KaiC, a core protein of the cyanobacterial circadian clock, consists of an N-terminal CI domain and a C-terminal CII domain, and assembles into a double-ring hexamer upon binding with ATP. KaiC rhythmically phosphorylates and dephosphorylates its own two adjacent residues Ser431 and Thr432 at the CII domain with a period of ∼24 h through assembly and disassembly with the other clock proteins, KaiA and/or KaiB. The core oscillator consists of the three kinds of proteins, KaiA, KaiB and KaiC and the clock can be reconstructed in vitro by mixing the three Kai-proteins with ATP. When co-incubated with KaiA and KaiB, KaiC exhibits circadian phosphorylation cycle as follows: ST → SpT → pSpT → pST → ST, where S, T, pS and pT represent S431, T432, phosphorylated S431 and phosphorylated T432, respectively.

In this study, we focused on an inner-radius side of the CII ring in KaiC as the research target based on our recent observation of KaiC crystal structures, in which an upstream region of the phosphorylation sites (T416-H429) at the inner-radius side undergoes a structural change. According to the crystal structures of KaiC, the side chain of F419 is oriented toward A422 and H423 on the neighboring protomer. We thus inserted a Trp residue at position 419 (KaiCF419W) to monitor the conformational change around the inner-radius side in solution by fluorescence spectroscopy. The F419W substitution had little impact on the overall structure of KaiC as evidenced by backbone RMSD of 0.42 Å between KaiCF419W and KaiCWT. Moreover, our biochemical assay demonstrated that KaiCF419W is virtually indistinguishable from KaiCWT in terms of clock function. Crystal structure of KaiCF419W-ST revealed that the indole ring of W419 was oriented toward the helical structure on the neighboring protomer. This suggests that the phospho-dependent variation of W419 fluorescence reflects the environmental change associated with the helix–coil transition. Although an interpretation of fluorescence from tryptophan in proteins is a challenging issue, one of the potential quenchers of W419 fluorescence on the basis of crystal structures of KaiC is a sulfur atom of M420. The side chain of W419 (or F419) is far from M420 in the ST state where the helical structure is formed, whereas they are in close proximity each other in the pSpT and pST states, in which the upstream region adopts the coil structure. Crystallographic analysis revealed that a side chain of Trp at the position of 419 was oriented toward a region undergoing a helix–coil transition, which is considered to be a key event to allosterically regulate the CI ring that plays a crucial role in determining the cycle period.

>MTSAEMTSPNNNSEHQAIAKMRTMIEGFDDISHGGLPIGRSTLVSGTSGTGKTLFSIQFLYNGIIEFDEPGVFVTFEETPQDIIKNARSFGWDLAKLVDEGKLFILDASPDPEGQEVVGGFDLSALIERINYAIQKYRARRVSIDSVTSVFQQYDASSVVRRELFRLVARLKQIGATTVMTTERIEEYGPIARYGVEEFVSDNVVILRNVLEGERRRRTLEILKLRGTSHMKGEYPFTITDHGINIFPLGAMRLTQRSSNVRVSSGVVRLDEMCGGGFFKDSIILATGATGTGKTLLVSRFVENACANKERAILFAYEESRAQLLRNAYSWGMDFEEMERQNLLKIVCAYPESAGLEDHLQIIKSEINDFKPARIAIDSLSALARGVSNNAFRQFVIGVTGYAKQEEITGLFTNTSDQWMGAHSITDSHISTITDTIILLQYVEIRGEMSRAINVFKMRGSWHDKAIREFMISDKGPDIKDSFRNFERIISGSPTRITVDEKSELSRIVRGVQEKGPES[2x]Strigolactones (SLs) and karrikins (KARs) are two classes of structurally related molecules that mediate signaling pathways to stimulate seed germination. SL and KAR have been reported to be recognized by the homologous proteins D14 (DWARF14)14–17 and HTL (HYPOSENSITIVE TO LIGHT; also known as KAI2, KARRIKIN INSENSITIVE2), respectively. To elucidate the structural basis of ligand specificity, we determined the crystal structures of ShHTL1, ShHTL4, ShHTL7, and ShD14 and compared their structures with those reported for ShHTL331 and ShHTL529. All the structures were highly similar to one another, consisting of a canonical α/β hydrolase domain and a helical cap.

ShHTL1 of the conserved clade is thought to be the ancestral ShHTL paralog. Only ShHTL1, in the conserved clade, was capable of binding KAR1 (dissociation constant (KD): 77 ± 12 μM; means ± standard deviation (SD), n = 3) with an affinity comparable to that of ShHTL3 of the intermediate clade (KD: 78 ± 3 μM). In contrast, ShHTL1 and ShHTL3 were KAR1 binding proteins without hydrolytic activity toward rac-GR24. In contrast, ShHTL1 and ShHTL3 showed no hydrolytic activity toward rac-GR24, while ShHTL1 had weak 5DS hydrolytic activity, which was so weak that 5DS-dependent germination was not observed in transgenic lines. The ligand-binding pocket of ShHTL1 (321 Å3) was composed of the largest number of bulky residues, resulting in a smaller pocket than AtHTL (411 Å3). Due to major bulky residues and the arrangement of the helix αD1, the pocket sizes of ShHTL1 and ShHTL3 were restricted so that there was only enough space to accommodate KAR. The structural alignment revealed that GR245DS might cause steric hindrance with L142, L/F190, and F194 of the KAR-binding proteins ShHTL1, ShHTL3, and AtHTL. Therefore, it is suggested that ShHTL1 interacts with ShMAX2 or AtMAX2 nonspecifically, while the interactions between AtHTL and ShMAX2 or AtMAX2 were induced in the presence of rac-GR24. Although the KD value for KAR binding of ShHTL1 (77 μM) was higher than the physiological concentration (1 μM), this result might be because the fraction of active protein in the sample was lower than 100%, resulting in lower estimated affinity than real affinity. Rather than the KAR receptor, ShHTL1 is likely to be the receptor for KL, an endogenous signaling molecule that shares structural similarity with KAR, in particular the butenolide ring.

>[2x]GPLGSMGLAQEAHNVRVLGSGPQTVVLAHGFGTDQSVWKYLVPHLVEDYRVVLFDIMGAGTTNPTYFNFERYSSLEGYAGDVIAILEELQISSCVYVGHSVSAMIGVIASVTRPDLFTKLVTVAGSPRYLNDPDYFGGFDLDELHELFEAMKENYKAWCSGFAPLCVGADMESLAVQEFSRTLFNMRPDIALSILQTIFYSDVRPLLPHVTVPCHIIQSVKDLAVPVAVSEYIHQSLGGESILEVMATEGHLPQLSSPDVVVPVLLRHIRYAIARPN> MRRNLRLGPSSGADAQGQGAPRPGLAAPRMLLP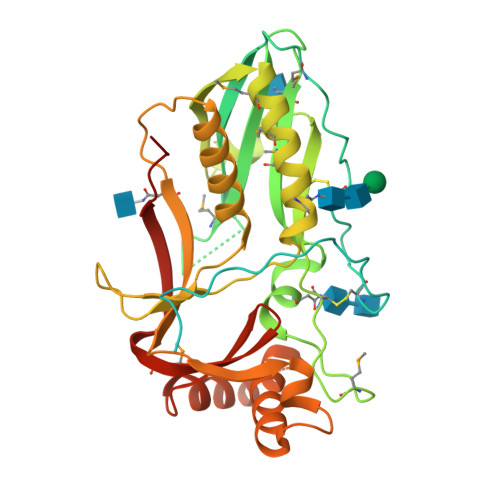PASQASRGSGSTGCSLMAQEVDTAQGAEMRRGAGAARGRASWCWALALLWLAVVPGWSRVSGIPSRRHWPVPYKRFDFRPKPDPYCQAKYTFCPTGSPIPVMEGDDDIEVFRLQAPVWEFKYGDLLGHLKIMHDAIGFRSTLTGKNYTMEWYELFQLGNCTFPHLRPEMDAPFWCNQGAACFFEGIDDVHWKENGTLVQVATISGNMFNQMAKWVKQDNETGIYYETWNVKASPEKGAETWFDSYDCSKFVLRTFNKLAEFGAEFKNIETNYTRIFLYSGEPTYLGNETSVFGPTGNKTLGLAIKRFYYPFKPHLPTKEFLLSLLQIFDAVIVHKQFYLFYNFEYWFLPMKFPFIKITYEEIPLPIRNKTLSGL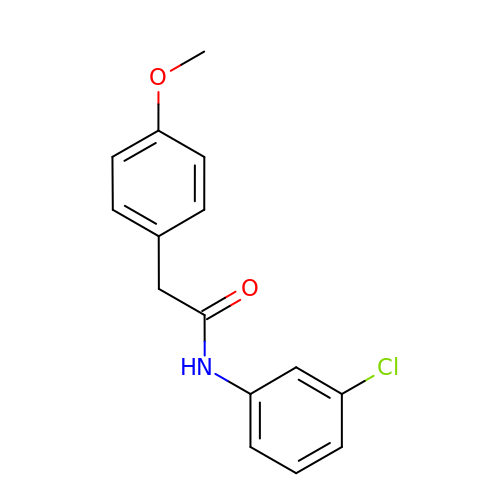N-(3-chlorophenyl)-2-(4-methoxyphenyl)acetamide | C15 H14 Cl N O2 | YWOVILWNVBQOEA-UHFFFAOYSA-N>GAAGLGHPAAFGRATHAVVRALPESLGQHALRSAKGEEVDVARAERQHQLYVGVLGSKLGLQVVELPADESLPDCVFVEDVAVVCEETALITRPGAPSRRKEVDMMKEALEKLQLNIVEMKDENATLDGGDVLFTGREFFVGLSKRTNQRGAEILADTFKDYAVSTVPVADGLHLKSFCSMAGPNLIAIGSSESAQKALKIMQQMSDHRYDKLTVPDDIAANCIYLNIPNKGHVLLHRTPEEYPESAKVYEKLKDHMLIPVSMSELEKVDGLLTCCSVLINKKVD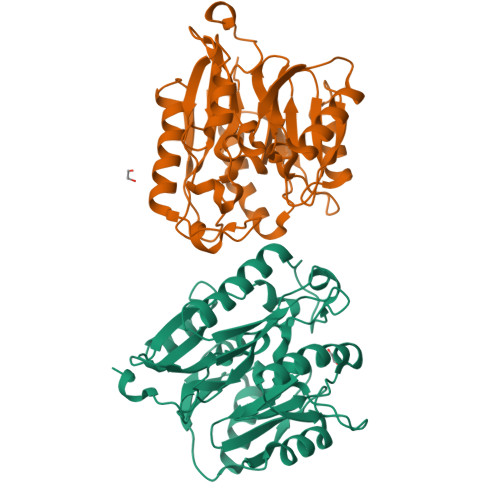S[2x]>MTKLITTVKEMQHIVKAAKRSGTTIGFIPTMGALHDGHLTMVRESVSTNDITIVSVFVNPLQFGPNEDFDAYPRQIDKDLELVSEVGADIVFHPAVEDMYPGELGIDVKVGPLADVLEGAKRPGHFDGVVTVVNKLFNIVMPD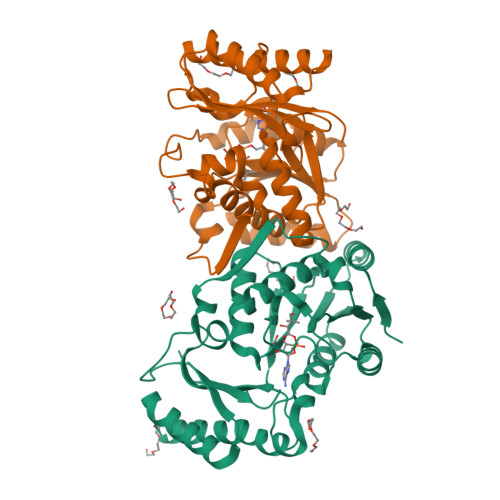YAYFGKKDAQQLAIVEQMVKDFNHAVEIIGIDIVREADGLAKSSRNVYLTEQERQEAVHLSKSLLLAQALYQDGERQSKVIIDRVTEYLESHISERIEEVAVYSYPQLVEQHEITGRIFISLAVKFSKARLIDNIIIGAE[2x]>GSHMARYDSLLQALGNTPLVGLQRLSPRWDDGRDGPHVRLWAKLEDRNPTGSIKDRPAVRMIEQAEADGLLRPGATILEPTSGNTGISLAMAARLKGYRLICVMPENTSVERRQLLELYGAQIIFSAAEGGSNTAVATAKELA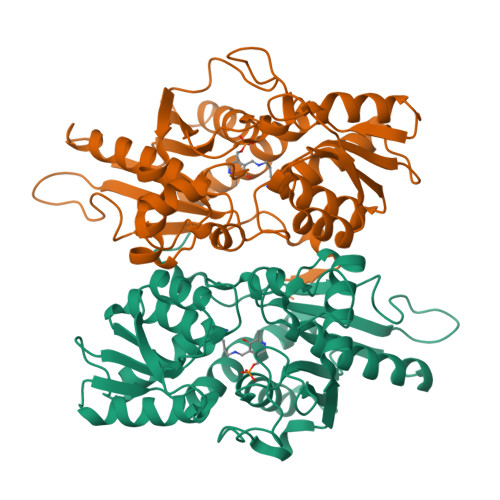ATNPSWVMLYQYGNPANTDSHYCGTGPELLADLPEITHFVAGLGTTGTLMGTGRFLREHVANVKIVAAEPRYGEGVYALRNMDEGFVPELYDPEILTARYSVGAVDAVRRTRELVHTEGIFAGISTGAVLHAALGVGAGALAAGERADIALVVADAGWKYLSTGAYAGSLDDAETALEGQLWA[2x]>SMLWNNKKDEHGPFDIIGDIHGCYDELKMLLEKLGYLIEEVEGGVGSGKYRVTHPEGRKVLFLGDLVDRGPKITEVLKLVMGMVKSGIALCVPGNHDVKLLRKLNGRDVQITHGLDRTLEQLAKEPQEFIEEVKAFIDGLVSHYVLDDGKLVVAHAGMKEEFQGRGSGKVREFALYGETTGETDEYGLPVRY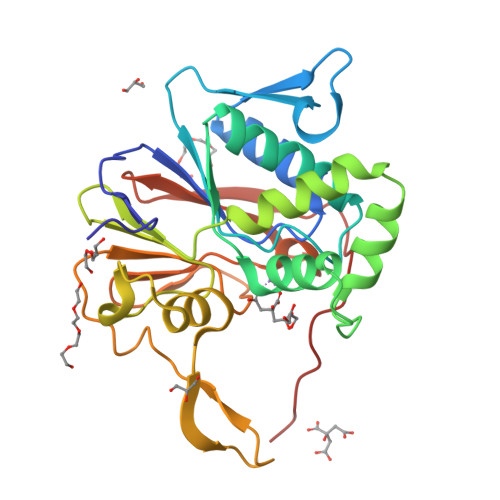DWASDYRGKALVVYGHTPQAEVLKVNNTINIDTGCVFGGKLTAYRYPEREIVDVKALKTYYEPALEHHHHHH[2x]>[4x]MSSVLASCPKKPVSSYLRFSKEQLPIFKAQNPDAKTTELIRRI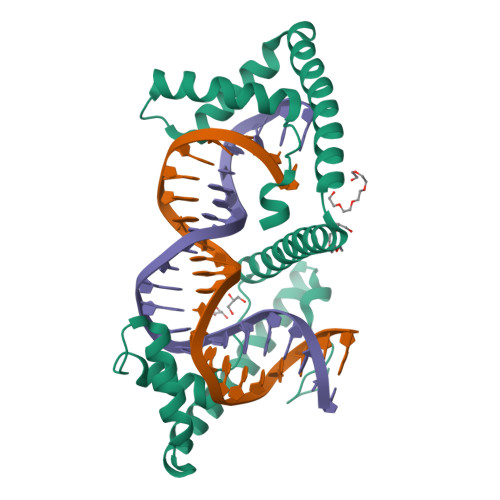AQRWRELPDSKKKIYQDAYRAEWQVYKEEISRFKEQLTPSQIMSLEKEIMDKHLKRKAMTKKKELTLLGKPKRPRSAYNVYVAERFQEAKGDSPQEKLKTVKENWKNLSDSEKELYIQHAKEDETRYHNEMKSWEEQMIEVGRKDLLRRTIKKQRKYGAEECLQHHHHHH>[3x]LTAKHRPSVVWLHNAECTGCTEAAIRTIKPYIDALILDTISLDYQETIMAAAGEAAEAALHQALEGKDGYYLVVEGGLPTIDGGQWGMVAGHPMIETTKKAAAKAKGIICIGTCSAYGGVQKAKPNPSQAKGVSEALGVKTINIPGCPPNPINFVGAVVHVLTKGIPDLDENGRPKLFYGELVHDNCPRLPHFEASEFAPSFDSEEAKKGFCLYELGCKGPVTYNNCPKVLFNQVNWPVQAGHPCLGCSEPDFWDTMTPFYEQG;>[3x]MAESKPTPQSTFTGPIVVDPITRIEGHLRIMVEVENGKVKDAWSSSQLFRGLEIILKGRDPRDAQHFTQRACGVCTYVHALASSRCVDDAVKVSIPANARMMRNLVMASQYLHDHLVHFYHLHALDWVDVTAALKADPNKAAKLAASIAPARPGNSAKALKA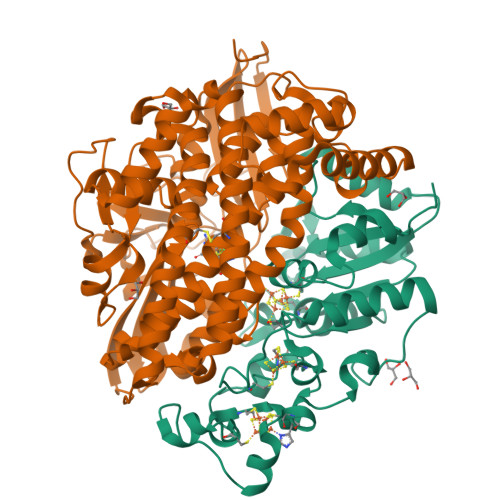VQDKLKAFVESGQLGIFTNAYFLGGHKAYYLPPEVDLIATAHYLEALHMQVKAASAMAILGGKNPHTQFTVVGGCSNYQGLTKDPLANYLALSKEVCQFVNECYIPDLLAVAGFYKDWGGIGGTSNYLAFGEFATDDSSPEKHLATSQFPSGVITGRDLGKVDNVDLGAIYEDVKYSWYAPGGDGKHPYDGVTDPKYTKLDDKDHYSWMKAPRYKGKAMEVGPLARTFIAYAKGQPDFKKVVDMVLGKLSVPATALHSTLGRTAARGIETAIVCANMEKWIKEMADSGAKDNTLCAKWEMPEESKGVGLADAPRGALSHWIRIKGKKIDNFQLVVPSTWNLGPRGAQGDKSPVEEALIGTPIADPKRPVEILRTVHAFDPCIACGVH> MSGTANSRRKEVLRVPVIDLNRVSDEEQLLPVVRAILLQHDTFLLKNYANKAVLDALLAGLTTKDLPDTSQGFDANFTGTLPLEDDVWLEQYIFDTDPQLRFDRKCRNESLCSIYSRLFKLGLFFAQLCVKSVVSSAELQDCISTSHYATKLTRY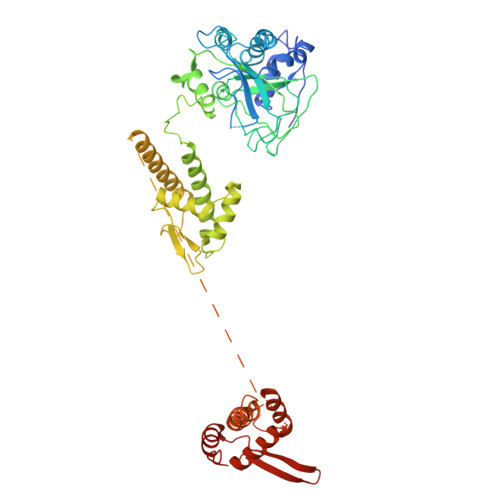FNDNGSTHDGADAGATVLPTGDDFQYLFERDYVTFLPTGVLTIFPCAKAIRYKPSTMATTDNSWVSIDEPDCLLFHTGTLLARWSQGMHTTSPLQIDPRANIVSLTIWPPLTTPISSKGEGTIANHLLEQQIKAFPKVAQQYYPRELSILRLQDAMKFVKELFTVCETVLSLNALSRSTGVPPELHVLLPQISSMMKRKIVQDDILKLLTIWSDAYVVELNSRGELTMNLPKRDNLTTLTNKSRTLAFVERAESWYQQVIASKDEIMTDVPAFKINKRRSSSNSKTVLSSKVQTKSSNANALNNSRYLANSKENFMYKEKMPDSQANLMDRLRERERRSAALLSQRQKRYQQFLAMKMTQVFDILFSLTRGQPYTETYLSSLIVDSLQDSNNPIGTKEASEILAGLQGILPMDISVHQVDGGLKVYRWNSLDKNRFSKLLQIHKSKQQD The African swine fever virus (ASFV) type II topoisomerase (Topo II), pP1192R, is the only known Topo II expressed by mammalian viruses and is essential for ASFV replication in the host cytoplasm. In ASFV, a functional viral Topo II pP1192R has been identified, encoded by a viral gene conserved in ASFV strains, P1192R. pP1192R is detectable at an intermediate to late stage of ASFV infection, mainly within the cytoplasmic virus factory, and has been confirmed to be important for ASFV replication. Topo IIAs exhibit a 2-fold symmetry and comprise two functional domains: an ATPase domain and a DNA binding/cleavage domain. The mechanism of enzymatic action involves the opening and closing of three gate-like dimeric interfaces, which are called the N-, DNA- and C-gate, respectively, upon ATP binding and hydrolysis and DNA cleavage that introduces a double-strand break in the DNA (G-segment) trapped in the DNA-gate for transport of another DNA strand (T-segment).

To capture the intact structure of full-length pP1192R, the protein sample was then analyzed by single-particle cryo-EM. After collecting and processing 2134 cryo-EM images, two types of particles, referred to as State 1 and State 2, were identified and reconstructed to the overall resolution of 2.77 and 2.98 Å with 131 161 and 78 195 particles, respectively. The electron density was only observable for the DNA binding/cleavage domain in both states, while the electron density of the N-terminal ATPase domain was absent. Following the process of atomic model building based on the EM density map, the apo structure of the pP1192R DNA binding/cleavage domain was well resolved in both states, with the C-terminus of the protein (C-gate) adopting distinct conformations, accordingly described as ‘open’ (State 1) and ‘closed’ (State 2). These apo structures can be traced for 779 residues, ranging from D416 to H1192, except for the region containing residues G471-N501. In the closed state, an extra dimeric interface, the C-gate, was formed by the interaction between the coiled-coil helices of two protomers, which retains a distance of ∼16 Å in the open state. No significant conformational changes were observed in the DNA-binding groove when comparing the two apo states, while the coiled-coil helices underwent a distinct conformational rearrangement, presenting the dynamic cycling of the C-gate between open to closed. The coiled-coil regions (from A' α14 to A' α18) of each protomer move towards one another in the closed state, with the furthest end moving a distance of ∼13.4 Å and a reorientation of ∼12° relative to the open state. Comparison of the m-AMSA-poisoned DNA-binding/cleavage domain with the apo structure (the C-gate closed state) revealed relative conformational reorientations of the DNA-contacting region of the two protomers.

>METFEISDFKEHAKKKSMWAGALNKVTISGLMGVFTEDEDLMALPIHRDHCPALLKIFDELIVNATDHERACHNKTKKVTYIKISFDKGVFSCENDGPGIPIVKHEQASLIAKRDVYVPEVASCYFLAGTNINKAKDCIKGGTNGVGLKLAMVHSQWAILTTADGSQKYVQHINQRLDNIEPPTITPSREMFTRIELMPVYQELGYAQPLSETEQADLSAWIYLRACQCAAYVGKGTTIYYNDKPCSTSSVMALAKMYTLVTAPNSTIYTATIKADAKPYSLHPLQVAAVVSPKFKKFEHVSIINGVNCVKGEHVTFLKKAINEMVVKKFQQTIKDKNRKTTLRDSCSNIFVVIVGSIPGIEWTGQRKDELSIAENVFKTHYSIPSSFLTSMTRSIVDILLQSISKKDNHKQIDVDKYTRARNAGGKKAQDCMLLAAEGDSALSLLRAGLTLGKSNPSGPSFDFCGMISLGGVIMNACKKVTNITTDSGETIMVRNEQLTNNKVLQGIVQVLGLDFNCHYKTQEERAKLRYGCIVACVDQDLDGCGKILGLLLAYFHLFWPQLIVHGFVKRLLTPLIRVYEKGNTVPVEFYYEQEFDAWAKKQTSLANHTVKYYKGLAAHDTHEVKSMFKHFDKMVYTFTLDDSAKELFHIYFGGESELRKRELCTGVVPLTETQTQSIHSVRRIPCSLHLQVDTKAYKLDAIERQIPNFLDGMTRARRKILAGGLKCFASNNRERKVFQFGGYVADHMFYHHGDMSLNTSIIKAAQYYPGSSHLYPVFIGIGSFGSRHLGGKDAGSPRYISVQLASEFIKTMFPTEDSWLLPYVFEDGQRAEPEYYVPVLPLAIMEYGANPSEGWKYTTWARQLEDILALVRAYVDKNNPKHELLHYAIDHKITVLPLRPSNYNFKGHLKRFGQYYYSYGTYVVSEQRNMITITELPLRVPTVAYIESIKKSSNRMAFIEEIVDYSSSETIEILVKLKPNSLSRIMEEFKETEEQNSIENFLRLRNCLHSHLNFVKPKGGIIEFNSYYEILYAWLPYRRDLYQKRLMRERAVLKLRLIMETAIVRYINESADLNLSHYEDEKEAGRILSEHGFPPLNQSLITSPEFATIEELNQKALQGCYTYILSLQARELLIAAKTRRVEKIKKMQARLDKVEQLLQESPFPGASVWLEEIDAVEKAIIKGRNTQWKFHHH[2x]>MFGKRDSSASGDPKAPPPAPAGGATIATRPQRVEPVAAPEPKAPAPKVSGPAPKPTVGLEQLRAAQGQPQTANIVREQSDYYHATKTTIFNALLNTIDLSQLAQLDLKQAGEEIRDIVAELVAIKNVSMSVAEQEHLVQDIINDVLGYGPLEPLLARDDIADIMVNGAHRVFIEVGGKVQLTNVRFRDNLQLMNICQRIVSQVGRRVDESSPICDARLPDGSRVNVIAPPLALDGPTLTIRKFKKDKLTMKNLVEFASISPEGARVLGVIGACRCNLVISGGTGSGKTTLLNTMTAFIDPTERVVTCEDAAELQLQQPHVVRLETRPPNLEGSGAVTMRDLVKNCLRMRPERIIVGEVRGPEAFDLLQAMNTGHDGSMGTLHANSPREAISRIESMITMGGYGLPSKTIKEMIVGSVDVIIQAARLRDGSRRITHITEVVGLEGDVIVTQDLFVYEITGEDEHGKVVGKHRSTGIARPRFWDRARYYGLERELAEALDAAE[6x]

The ATPase CpaF in C. crescentus is the only Tad motor reported to date that is known to be bifunctional, facilitating both pilus extension and retraction at the flagellar pole through ATP hydrolysis. CpaF oligomerization is mediated by interactions between the NTD of one chain and the CAD of an adjacent chain. From these data, we propose that CpaF uses a clockwise, rotary mechanism of catalysis to assemble a right-handed, helical Tad pilus, a process broadly applicable to other single motor systems.

Saturating all nucleotide binding sites with excess ATP yielded another expanded structure at a global resolution of 3.3 Å. All particles contributed to the single reconstruction, and the nucleotide composition was identical to the expanded structure from the under-saturated dataset. The presence of ADP, despite supplementing the sample with excess ATP, suggests purified CpaF harbors in vitro enzymatic activity. The expanded hexamers in the two different datasets superimpose with an RMSD of 1.5 Å. Increasing nucleotide concentrations favor the expanded state. Since CpaF assumes three main conformations in a nucleotide-dependent manner, we believe the closed, compact, and expanded states captured in the apo, under-saturating, and saturating datasets, respectively, best represent the catalytic cycle. Given the expanded state harbors two ADP-bound monomers in the asymmetric unit, we further classify Exp-ADP into Exp-ADP1 and Exp-ADP2. In summary, the coupling of ATP binding and hydrolysis expands the hexamer and rotates the C2 axis clockwise by 60°. The predicted C3-symmetric CpaGH heterotrimer fits snugly into the hexamer pore of the CpaF expanded state, suggesting that in this ATPase conformation, the platform complex could facilitate entry of three pilin subunits from the inner membrane into the central platform shaft through the openings between CpaGH heterodimers, gated by the N-terminal α1 of CpaH.4-{[(2S)-2-(1,3-dioxo-1,3-dihydro-2H-isoindol-2-yl)propyl]oxy}-3,5-dimethylphenyl 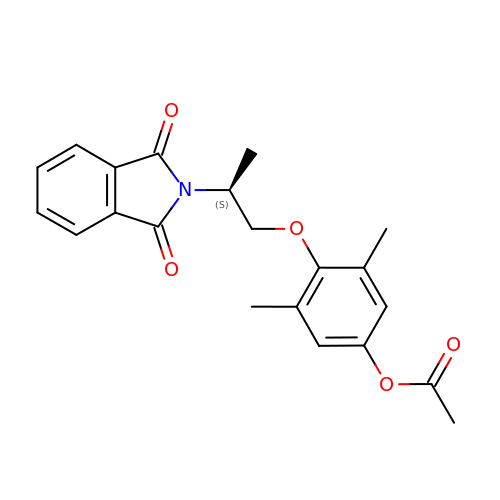acetate | C21 H21 N O5 | UICXIWCGDWFHDK-AWEZNQCLSA-N> SMKINFLRNKHKIHVQGT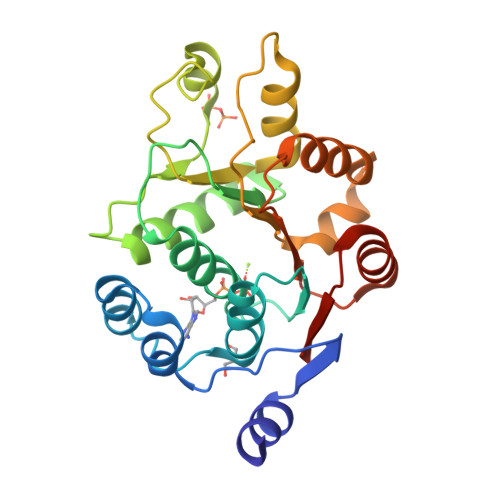DLPDPIATFQQLDQEYKINSRLLQNILDAGFQMPTPIQMQAIPVMLHGRELLASAPTGSGKTLAFSIPILMQLKQPANKGFRALIISPTRELASQIHRELIKISEGTGFRIHMIHKAAVAAKKFGPKSSKKFDILVTTPNRLIYLLKQDPPGIDLASVEWLVVDESDKLFEDGKTGFRDQLASIFLACTSHKVRRAMFSATFAYDVEQWCKLNLDNVISVSIGARNS>[2x]DEKTVQRYYKTTVPTKPKKPHDISAFVKSALPHLSFVVLGHV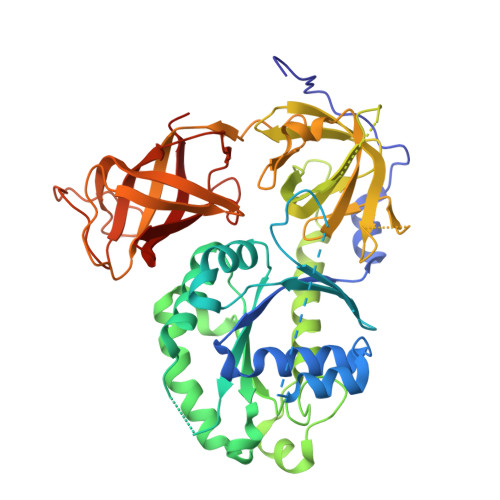DAGKSTLMGRLLYDLNIVNQSQLRKLQRESETMGKSSFKFAWIMDQTNEERERGVTVSICTSHFSTHRANFTIVDAPGHRDFVPNAIMGISQADMAILCVDCSTNAFESGFDLDGQTKEHMLLASSLGIHNLIIAMNKMDNVDWSQQRFEEIKSKLLPYLVDIGFFEDNINWVPISGFSGEGVYKIEYTDEVRQWYNGPNLMSTLENAAFKISKENEGINKDDPFLFSVLEIIPSKKTSNDLALVSGKLESGSIQPGESLTIYPSEQSCIVDKIQVGSQQGQSTNHEETDVAIKGDFVTLKLRKAYPEDIQNGDLAASVDYSSIHSAQCFVLELTTFDMNRPLLPGTPFILFIGVKEQPARIKRLISFIDKGNTASKKKIRHLGSKQRAFVEIELIEVKRWIPLLTAHENDRLGRVVLRKDGRTIAAGKISEITQHHHHHH>[4x]MKMDKKTIVWFRRDLRIEDNPALAAAAHEGSVFPVFIWCPEEEGQFYPGRASRWWMKQSLAHLSQSLKALGSD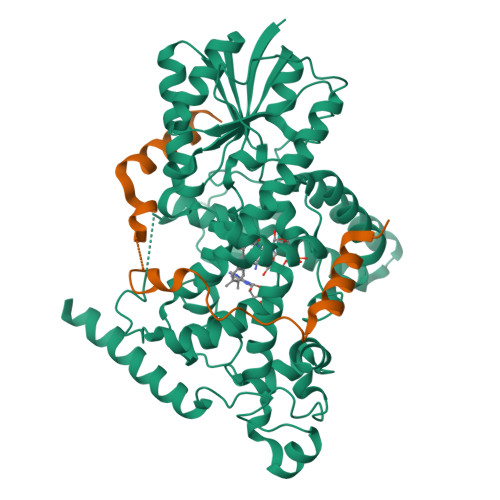LTLIQTHNTISAILDCIRVTGPTKVVFNHLYDPVSLVRDHTVKEKLVERGISVQSYNGDLLYEPWEIYCEKGKPFTSFNSYWKKCLDMSIESVMLPPPWRLMPITAAAEAIWACSIEELGLENEAEKPSNALLTRAWSPGWSNADKLLNEFIEKQLIDYAKNSKKVVGNSTSLLSPYLHFGEISVRHVFQCARMKQIIWARDKNSEGEESADLFLRGIGLREYSRYICFNFPFTHEQSLLSHLRFFPWDADVDKFKAWRQGRTGYPLVDAGMRELWATGWMHNRIRVIVSSFGVKFLLLPWKWGMKYFWDTLLDADLECDILGWQYISGSIPDGHELDRLDNPALQGAKYDPEGEYIRQWLPELARLPTEWIHHPWDAPLTVLKASGVELGTNYAKPIVDIDTARELLAKAISRTREAQIMIGAAPDEIVADSFEALGANTIKEPGLCPSVSSNDQQVPSVVRYNGSKRVKPEEEEERDMKKSRGFDERELFSTAESSSSSSVFFVSQSCSLASEGKNLEGIQDSSDQITTSLGKNGCK;>PETTVLSGRDRLKRHREEVAGKVPIPDSWGKEGLLMGWMDFSTFDAAFTSSQIVSARAALMADSGHHHHHH[4x]>[2x]MPEVVFGSTYTKGKIA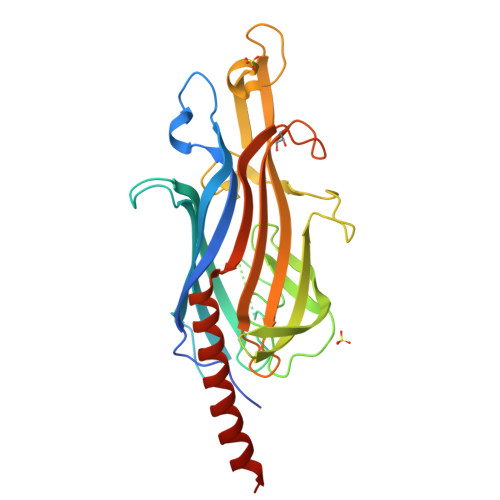KIPLDIDTSLVSDGTATAFDPDSLVAERFKIDRDVPVALQQQMSVEAPSNADVVTFQVGTTLRRTDRQQDAGLLLALVDTVTMNRNTAEAVSSENNPGGAVQKPRAIEDEKPPTNIALPHEGLTYRFPFDTEKKTYPFFDPIAQKAFDANYDGEEDVNGLTTYRFVQNVGYDADGKLADPIKYSSLYEDDADASVTARAEVWGVPGEPDESITMDRFYAASRTFWVDPVSGTIVKSEEHGYQYYAREALKPEVTYVDFKVTTNEESVESQVAAASDERDRIALWTRSRHHHHHH> GGIVVYWGQNGGEGTLTSTCESGLYQIVNIAFLSQFGGGRRPQINLAGHCDPANNGCRTVSDGIRACQRRGIKVMLSIGGGAGSYSLSSVQDARSVADYIWNNFLGGRSSSRPL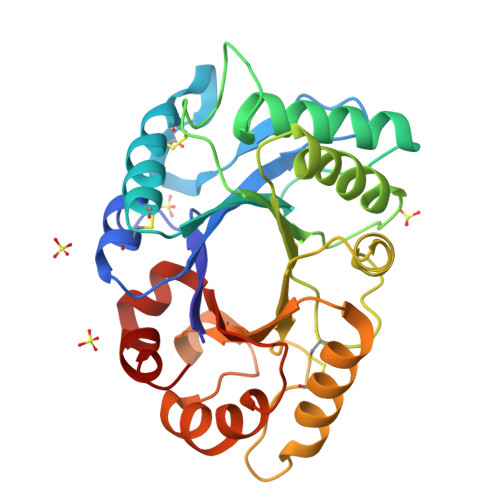GDAVLDGVDFDIEHGGAYYDALARRLSEHNRGGKKVFLSAAPQCPFPDQSLNKALSTGLFDYVWVQFYNNPQCEFNSGNPSNFRNSWNKWTSSFNAKFYVGLPASPEAAGSGYVPPQQLINQVLPFVKRSPKYGGVMLWDRFNDLKTKYSSKIKPSV> GFPTELKPGTNQFLTTDDGVSAPILPNFHPTPCIHIPGEVRNLLELCQVETILEVNNVPTNATSLMERLRFPVSAQAGKGELCAVFRADPGRDGPWQSTMLGQLCGYYTQWSGSLEVTFMFTGSFMATGKMLIAYTPPGGPLPKDRATAMLGTHVIWDFGLQSSVTLVIP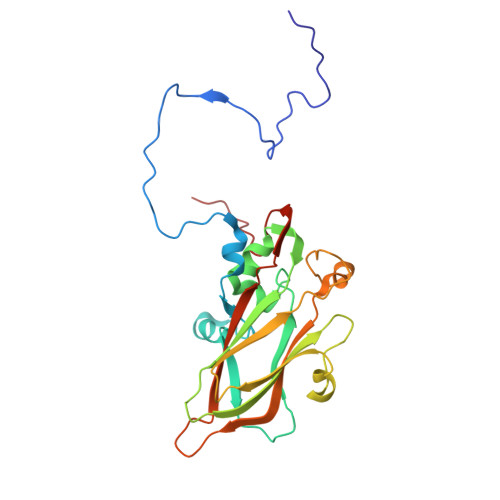WISNTHYRAHARDGVFDYYTTGLVSIWYQTNYVVPIGAPNTAYIIALAAAQKNFTMKLCKDTSHILQTASIQ4-amino-N-(6-methoxypyrimidin-4-yl)benzene-1-sulfonamide 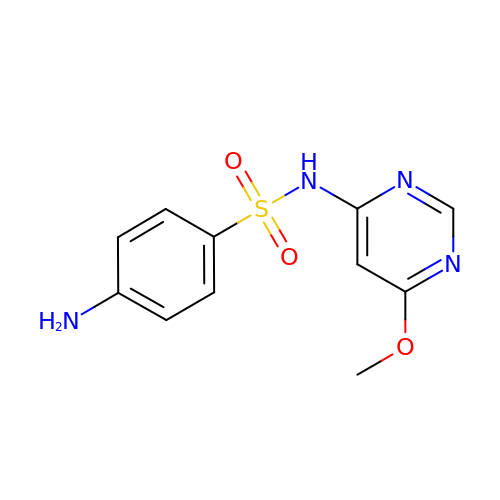| C11 H12 N4 O3 S | WMPXPUYPYQKQCX-UHFFFAOYSA-N> MPLKAYRPPEDPGLWDTYLEWLERALKVAGVHPTTLEYLAHPKRLVTLSLPVVMDDGKVRIFQGYRVVHDIARGPAKGGVRLDPGVTLGQTAGLAAWMTLKAAVYDLPFGGAAGGIAVDPKGLSPQELERLVRRYTAELVGLIGPDSDILGPDLGADQQVMAWIMDTYSM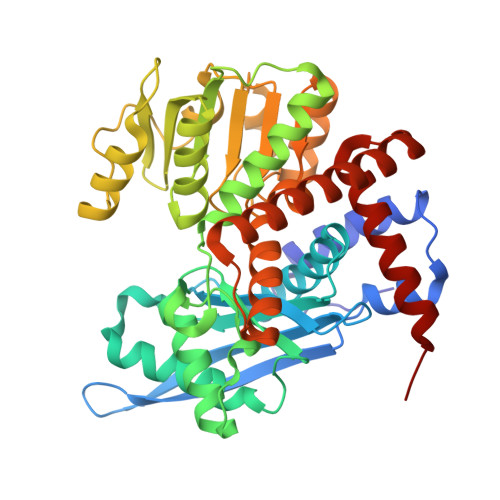TVGSTVPGVVTGKPHALGGSEGRDDAAGLGALLVLEALAKRRGLDLRGARVVVQGLGQVGAAVALHAERLGMRVVAVATSMGGMYAPEGLDVAEVLSAYEATGSLPRLDLAPEEVFGLEAEVLVLAAREGALDGDRARQVQAQAVVEVANFGLNPEAEAYLLGKGALVVPDLLSGGGGLLASYLEWVQDLNMFFWSPEEVRERFETRVARVVDAVCRRAERGGLDLRMGALALALERLDEATRLRGVYP> XTIVALKYPGGVVMAGDRRSTQGNMISGRDVRKVYITDDYTATGIAGTAAVAVEFARLYAVELEHYEKLEGVPLTFAGKINRLAIMVRGNLAAAMQGLLALPLLAGYDIHASDPQSAGRIVSFDAAGGWNIEEEGYQAVGSG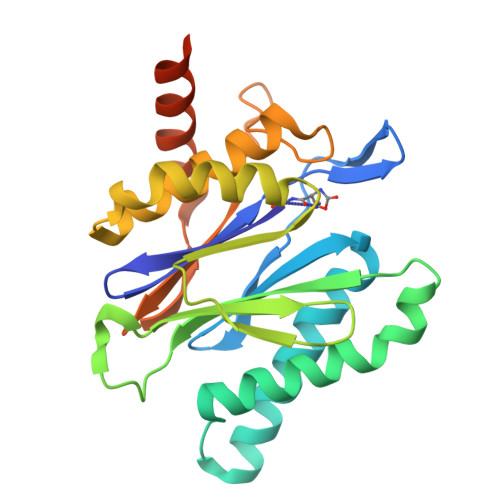SLFAKSSMKKLYSQVTDGDSGLRVAVEALYDAADDDSATGGPDLVRGIFPTAVIIDADGAVDVPESRIAELARAIIESRSGADTFGSDGGEKHHHHHH2-[(3aS,7aR)-2-amino-3a-(2,4-difluorophenyl)-3a,6,7,7a-tetrahydro[1,3]oxazolo[4,5-c]pyridin-5(4H)-yl]pyridine-3-carbonitrile | C18 H15 F2 N5 O | 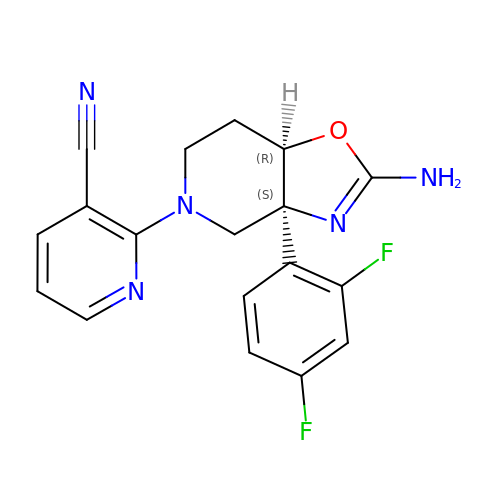UKQSZNNDBLMQNX-CRAIPNDOSA-N> KRAALIQNLRD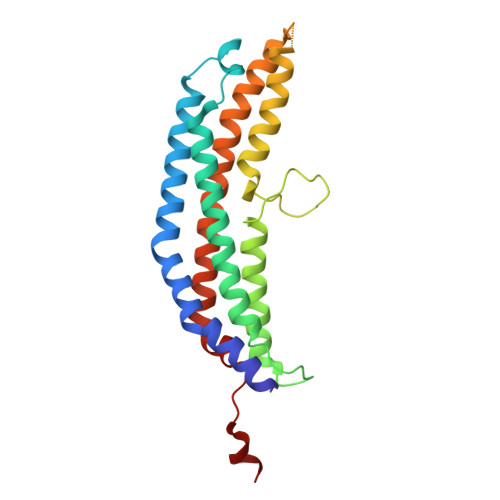SYTETSSFAVIEEWAAGTLQEIEGIAKAAVEAHGTIRNSTYGRAQAEKSPEQLLGVLQRYQDLCHNVYCQAETIRTVIAIRIPEHKEADNLGVAVQHAVLKVIDELEIKTLGSGEKSGSGGAPTPIGMYALREYLSARSTVEDKLLGSVDAESGKTKGGSQSPSLLLELRQIDADFMLKVELATTHLSTMVRAVINAYLLNWKKLIQPRGGHLDVLYR(2R)-2-methylbutanedioic acid | C5 H8 O4 | 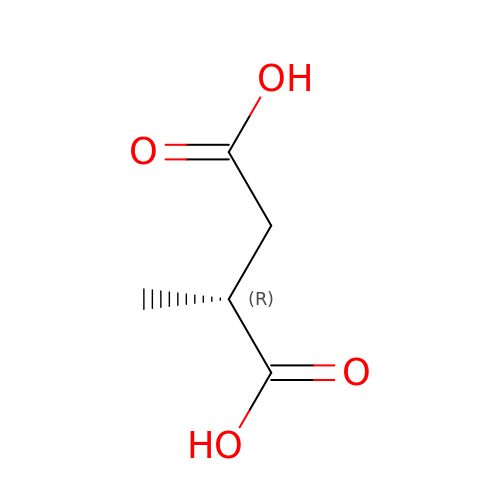WXUAQHNMJWJLTG-GSVOUGTGSA-N[bis(chloranyl)-[oxidanyl-[(2~{E},6~{E})-3,7,11-trimethyldodeca-2,6,10-trienoxy]phosphoryl]methyl]phosphonic 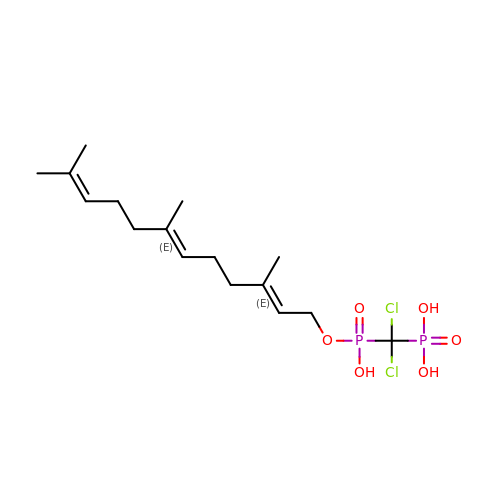acid | C16 H28 Cl2 O6 P2 | SCZVAQFGXARGRA-YFVJMOTDSA-N We have investigated the function and structure of Trichodesmium Tery_3377, an iron stress-induced protein (iron deficiency-induced A, IdiA) commonly used as an in situ marker of iron stress. Using heterologous expression in the model cyanobacteria Synechocystis PCC6803, we provide evidence that Tery_3377, a commonly used iron-limitation biomarker, is localized to the periplasm with a suggested FutA2 function as an iron-binding protein of an ABC transporter. The overall fold of Tery_3377 assumes a classic small molecule ABC transporter substrate-binding domain fold, with two domains hinged over a substrate-binding cleft. The hinge region is formed by two short β-strands and connects the protein domains via a double cross-over between the N (residues 34–133 and 266–349) and C termini (134–265). This type of structure places Tery_3377 among class IV iron-binding proteins (in keeping with Ref. 27) and allows for structural classification within cluster D of the substrate-binding domains.

To try and crystalline ligand-free Tery_3377 to examine structural changes upon iron binding, we citrate-treated Tery_3377 protein preparations prior to crystallization; citrate is known to chelate iron and was added to remove all iron from the protein preparation. Additional support for the plasticity in the binding of Tery_3377 comes from the observation of bound citrate in the binding cleft, clearly indicating the potential for binding of organic compounds. It is interesting to speculate that binding of organic ligands together with iron may represent a mechanism of siderophore recognition. The structural data further show a remarkable plasticity of the substrate-binding cleft, allowing organic molecules and potentially siderophores to bind in addition to Fe3+.

>[2x]GAINLYSSRHYDTDQALYDSFTKKTGLKVNLIEGKGDKLIERIKSEGANSPADVFMTVDAGRLWRAQEAGILQPISSSTLNNKIPANLRSPEKLWFGFSKRARVIMYNKNKVQPSELSTYEDLAQNKWKGKIVIRSSSNIYNQSLIASLIEIHGMSDAEGWAKGFVRNFARPPEGNDTAQIKAVAAGIGDIGLANSYYLARLKRSSKPEDQAVADKVGMFFPNQNGRGTHVNISGGGVVKNAPNKEGAIKFLEYLVSPEAQKIFSEGNNEYPVVAGVPIASVLKPFGSFKNDSTNVSVYGKLNADAIKLMDRVGWKLE> HHHHHHPPCETHETGTTNTATTATGGGTHADSLNNLANIKREQGNIEEAVRLYRKALEVFPEFAAAHSNLASVLQQQGKLQEALMHYKEAIRISPTFADAYSNMGNTLKEMQDVQGALQCYTRAIQINPAFADAHSNLASIHKDSGNIPEAIASYRTALKLKPDFPDAYCNLAHCLQIVCDWTDYDERMKKLVSIVADQLEKNRLPSVHPHHSMLYPLSHGFRKAIAERHGNLCLDKINVLHKPPYEHPKDLKLSDGRLRVGYVSSDFGNHPTSHLMQSIPGMHNPDKFEVFCYALSPDDGTNFRVKVMAEANHFIDLSQIPCNGKAADRIHQDGIHILVNMNGYTKGARNELFALRPAPIQAMWLGYPGTSGALFMDYIITDQETSPAEVAEQYSEKLAYMPHTFFIGDHANMFPHLKKKAVIDFKSNGHIYDNRIVLNGIDLKAFLDSLPDVKIVKMKCPDGGDNADSSNTALNMPVIPMNTIAEAVIEMINRGQIQITINGFSISNGLATTQINNKAATGEEVPRTIIVTTRSQYGLPEDAIVYCNFNQLYKIDPSTLQMWANILKRVPNSVLWLLRFPAVGEPNIQQYAQNMGLPQNRIIFSPVAPKEEHVRRGQLADVCLDTPLCNGHTTGMDVLWAGTPMVTMPGETLASRVAASQLTCLGCLELIAKNRQEYEDIAVKLGTDLEYLKKVRGKVWKQRISSPLFNTKQYTMELERLYLQMWEHYAAGNKPDHMIKPVEVTESA

Remarkably, this modification is regulated by only two antagonistic enzymes: the O-GlcNAc transferase (OGT), which transfers the GlcNAc moiety onto acceptor residues from the donor sugar nucleotide UDP-GlcNAc, and the O-GlcNAc hydrolase (OGA), which removes it. OGT is a multi-domain protein with a catalytic core at the C-terminus and 13 tetratricopeptide (TPR) repeats at the N-terminus, making up about half of the enzyme. Here, we exploit a novel approach to covalently trap OGT-substrate complexes to explore how OGT recognizes glycosylation substrates through its TPR domain. Here, we used a fusion approach to trap OGT-substrate complexes to investigate the role of the TPRs in recognition of glycosylation substrates.

HCF1 is initially expressed as an approximately 210 kDa protein that is activated by limited proteolysis (protease maturation) within the proteolytic processing domain (PPD), consisting of multiple 20-residue repeats. A depletion of OGT leads to an accumulation of full-length HCF1 protein and the PPD is proteolytically cleaved by OGT via an unusual glycosylated glutamate intermediate. In the OGT:HCF1PRO structure, the peptide substrate spans the whole length of the TPR domain. The peptide interacts with the TPRs through some of its side chains, but intriguingly five regularly spaced asparagine side chains in OGT form hydrogen bonds with the HCF1PRO peptide backbone in a sequence-independent manner. We noted the fortuitous proximity of the HCF1PRO C-terminus to the OGT N-terminus (CαHCF1–1340-CαOGT313 approx. 12 Å), and wondered whether this would enable the direct tethering of substrates to OGT via a fusion linker to allow us to explore OGT-glycosylation substrate complexes. We first demonstrated that this fusion approach recapitulates the published HCF1PRO peptide binding mode and then used that to reveal how the C-terminus of the OGT glycosylation substrate TAB1 is recognized by the enzyme. Remarkably, this is also similar to the proteolytic cleavage site of a HCF1PRO repeat, with the major difference being a glutamate at the acceptor position. PCR primers (6H_HCF1_GGG_hOGT_fwd GTATTCATGCATCATCACCACCATCACccgccctgcgagacccacg, 6H_HCF1_GGG_hOGT_rev CAGGTTGTTCAGGGAATCAGCATGGGTaccgccaccggtggcggtggtggcggtg; 6H_TAB1_GGG_hOGT_fwd GTATTCATGCATCATCACCACCATCACGTGCCATACTCCAGCGCCCAG and 6H_TAB1_GGG_hOGT_rev CAGGTTGTTCAGGGAATCAGCATGGGTaccgccaccAAGGGAGAGGGTCACGCTGGTC) were then designed to introduce a TAB1 or HCF1 peptide followed by a GGG linker in place of the PreScission Protease site and the first two residues of the hOGT, changing the boundaries to 315–1031. Crystals grew in 2–3 days in 3.5 M sodium formate, 0.1 M Tris pH 8.5 for TAB1-OGT fusion and 1.3 M ammonium tartrate dibasic, 0.1 M Tris pH 8.5 for HCF1PRO:OGT. Crystals belong to space groups P6122 (TAB1:OGT) and P6222 (HCF1PRO:OGT) and have one molecule per asymmetric unit.SARS-CoV-2 is a positive-strand RNA virus. Its replication is mediated by a multisubunit replication-and-transcription complex of viral nonstructural proteins (nsps). The core component of this complex is the catalytic subunit (nsp12) of an RNA-dependent RNA polymerase (RdRp). By itself, nsp12 has little activity and its functions require accessory factors, including nsp7 and nsp8 (14, 15), that increase RdRp template binding and processivity.

The structure of the template-RTP RdRp complex contains one nsp12, one nsp7, and one nsp8. The overall structure of the template-RTP RdRp complex is similar to the apo RdRp structure, with nsp12 in a closed conformation. The double-stranded RNA helix, formed by 11 base pairs from the template-primer RNA, is held by the finger-palm-thumb subdomains. Extensive protein-RNA interactions are observed between the template-primer RNA and nsp12, with a total of 41 residues from nsp12 directly participating in RNA binding (within 4.0 Å of RNA, 26 residues to the template strand and 15 residues to the primer strand). There are no contacts from nsp12 to any base pairs of the template-primer RNA, suggesting a sequence-independent binding of RNA by RdRp. Despite the presence of excess RTP in complex assembly, only a single RMP is assembled into the primer strand, as observed in the structure. The RMP position is at the center of the catalytic active site. In addition, RMP forms interactions with side chains from K545 and R555. Near the bound RMP are two magnesium ions and a pyrophosphate. The pyrophosphate is at the gate of the nucleotide entry channel to the active site and may block the entry of nucleotide triphosphate to the active side.

> MSADAQSFLNRVCGVSAARLTPCGTGTSTDVVYRAFDIYNDKVAGFAKFLKTNCCRFQEKDEDDNLIDSYFVVKRHTFSNYQHEETIYNLLKDCPAVAKHDFFKFRIDGDMVPHISRQRLTKYTMADLVYALRHFDEGNCDTLKEILVTYNCCDDDYFNKKDWYDFVENPDILRVYANLGERVRQALLKTVQFCDAMRNAGIVGVLTLDNQDLNGNWYDFGDFIQTTPGSGVPVVDSYYSLLMPILTLTRALTAESHVDTDLTKPYIKWDLLKYDFTEERLKLFDRYFKYWDQTYHPNCVNCLDDRCILHCANFNVLFSTVFPPTSFGPLVRKIFVDGVPFVVSTGYHFRELGVVHNQDVNLHSSRLSFKELLVYAADPAMHAASGNLLLDKRTTCFSVAALTNNVAFQTVKPGNFNKDFYDFAVSKGFFKEGSSVELKHFFFAQDGNAAISDYDYYRYNLPTMCDIRQLLFVVEVVDKYFDCYDGGCINANQVIVNNLDKSAGFPFNKWGKARLYYDSMSYEDQDALFAYTKRNVIPTITQMNLKYAISAKNRARTVAGVSICSTMTNRQFHQKLLKSIAATRGATVVIGTSKFYGGWHNMLKTVYSDVENPHLMGWDYPKCDRAMPNMLRIMASLVLARKHTTCCSLSHRFYRLANECAQVLSEMVMCGGSLYVKPGGTSSGDATTAYANSVFNICQAVTANVNALLSTDGNKIADKYVRNLQHRLYECLYRNRDVDTDFVNEFYAYLRKHFSMMILSDDAVVCFNSTYASQGLVASIKNFKSVLYYQNNVFMSEAKCWTETDLTKGPHEFCSQHTMLVKQGDDYVYLPYPDPSRILGAGCFVDDIVKTDGTLMIERFVSLAIDAYPLTKHPNQEYADVFHLYLQYIRKLHDELTGHMLDMYSVMLTNDNTSRYWEPEFYEAMYTPHTVLQGGSENLYFQGHHHHHHHH;> MAIASEFSSLPSYAAFATAQEAYEQAVANGDSEVVLKKLKKSLNVAKSEFDRDAAMQRKLEKMADQAMTQMYKQARSEDKRAKVTSAMQTMLFTMLRKLDNDALNNIINNARDGCVPLNIIPLTTAAKLMVVIPDYNTYKNTCDGTTFTYASALWEIQQVVDADSKIVQLSEISMDNSPNLAWPLIVTALRANSAVKLQHHHHHHHH;> MSKMSDVKCTSVVLLSVLQQLRVESSSKLWAQCVQLHNDILLAKDTTEAFEKMVSLLSVLLSMQGAVDINKLCEEMLDNRATLQHHHHHHHH> AANDNNVEWNGLFHDQGPLFDNAPEPTSTQSVTLKLRTFKGDITSANIKYWDTADNAFHWVPMVWDSNDPTGTFDYWKGTIPASPSIKYYRFQINDG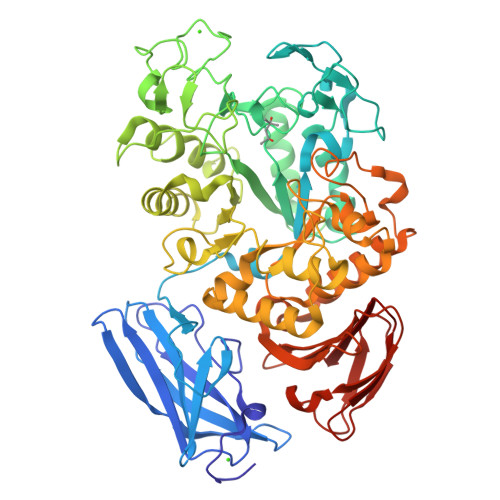TSTAWYNGNGPSSTEPNADDFYIIPNFKTPDWLKNGVMYQIFPDRFYNGDSSNDVQTGSYTYNGTPTEKKAWGSSVYADPGYDNSLVFFGGDLAGIDQKLGYIKKTLGANILYLNPIFKAPTNHKYDTQDYMAVDPAFGDNSTLQTLINDIHSTANGPKGYLILDGVFNHTGDSHPWFDKYNNFSSQGAYESQSSPWYNYYTFYTWPDSYASFLGFNSLPKLNYGNSGSAVRGVIYNNSNSVAKTYLNPPYSVDGWRLDAAQYVDHQIWSEFRNAVKGVNSNAAIIGEYWGNANPWTAQGNQWDAATNFDGFTQPVSEWITGKDYQNNSASISTTQFDSWLRGTRANYPTNVQQSMMNFLSNHDITRFATRSGGDLWKTYLALIFQMTYVGTPTIYYGDEYGMQGGADPDNRRSFDWSQATPSNSAVALTQKLITIRNQYPALRTGSFMTLITDDTNKIYSYGRFDNVNRIAVVLNNDSVSHTVNVPVWQLSMPNGSTVTDKITGHSYTVQNGMVTVAVDGHYGAVLAQ> GSHMGFKSGIDLLKQRSTVWKLSTSSSELDSVLGGGLESQSVTEFAGVFGSGKTQIMHQSCVNLQNPEFLFYDEEAVSKGEVAQPKAVYIDTEGTFRPER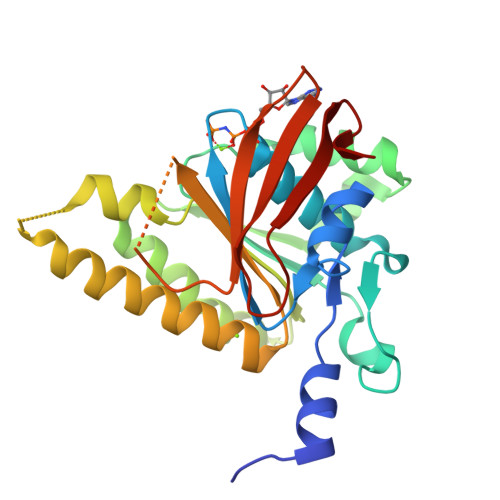IMQMAEHAGIDGQTVLDNTFVARAYNSDMQMLFAEKIEDLIQEGNNIKLVVIDSLTSTFRNEYTGRGKLAERQQKLGRHMATLNKLADLFNCVVLVTNQVSAKPDAFFGMAEQAIGGHIVGHAATFRFFVRKGKGDKRVAKLYDSPHLPDAEAIFRITEKGIQD> XF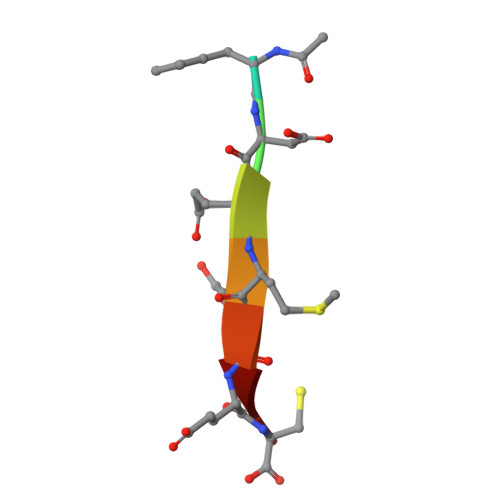DEMEEC Transcription termination is an essential step in transcription by RNA polymerase (RNAP) and crucial for gene regulation. For many bacterial genes, transcription termination is mediated by the adenosine triphosphate–dependent RNA translocase/helicase Rho, which causes RNA/DNA dissociation from the RNAP elongation complex (EC). Rho is an adenosine triphosphate (ATP)–dependent RNA translocase/helicase with 5′ → 3′ directionality. Rho forms a ring-shaped homo-hexameric complex, mediated by the CTD.

The type 1 and type 2 RNAP-Rho complexes both revealed the closed-ring Rho hexamer with RNA threaded in the central channel, but they have different Rho binding sites and orientations relative to RNAP. Our cryo-EM analysis also provided another Rho-RNAP complex (the type 2 complex), in which Rho binds near the DNA exit site of apo RNAP through its NTD side. In the type 2 complex, Rho is bound to RNAP in an inverted orientation, as compared with that in the type 1 complex. The Rho hexamer assumes a closed-ring conformation with RNA threaded through the Rho central channel and binds near the DNA exit site of RNAP through its NTD side. Four of the six Rho protomers are involved in the RNAP interaction: Rho protomers B and C contact the base part of the β-flap domain (residues β727 to β738), protomers C and D contact the jaw-lobe 1 domain, and protomer E contacts the clamp coiled-coil of RNAP. The T4L insertions into the NTD did not affect the RNA release activity of Rho. Moreover, the deletion of the RNAP β-flap tip, which is critical for the Rho-dependent RNA release, enhanced the formation of the type 2 complex. Therefore, the inverted Rho-binding mode in this complex is unlikely to be relevant to termination. The abundance of the type 2 complex in the cryo-EM particles suggests that Rho may preferentially bind apo RNAP in this alternative mode. Therefore, this complex could potentially resemble a posttermination state formed after the EC has released DNA and RNA.

>[6x]GPMRRKETLQETPLTYQELASKILPELHLLAQEAGIEGYKRMKKDQLIMALLERQTQGEGLRLVKGYLEISQDGYGFLTENLHNLESRVAIVSAGLIKQYALRAGDYVVGQARPPRENERYATLLKVEAVNNLDPEAAKNRPRFDELTPQFPDRQIRLETTPDELSTRVIDLLAPIGRGQRGLIVAPPKAGKTTLLKKIANAVLKNEPDIKVIVLLIDERPEEVTDFRESVQGAEVIASTFDEPPQNHIRVAEFVHERAKRIVEEGGHVMILLDSITRLARANNLVTPPTGRTLSGGLDSAALYFPKRFLGAARNIRGGGSLTILATALVETGSRMDDVIFEEFKGTGNMELHLSRRLEERRIFPAIDILKSGTRREELLLGEEVTHKMWLLRKVLADMDPAEAMEMLLARLARTKNNKEFLASLAAR;>[2x]MLDSKLKAPVFTVRTQGREYGEFVLEPLERGFGVTLGNPLRRILLSSIPGTAVTSVYIEDVLHEFSTIPGVKEDVVEIILNLKELVVRFLNPSLQTVTLLLKAEGPKEVKARDFLPVADVEIMNPDLHIATLEEGGRLNMEVRVDRGVGYVPAEKHGIKDRINAIPVDAVFSPVRRVAFQVEDTRLGQRTDLDKLTLRIWTDGSVTPLEALNQAVEILREHLTYFSNPQAAAVAAPEEAKEPEAPPEQEEELDLPLEELGLSTRVLHSLKEEGIESVRALLALNLKDLKNIPGIGERSLEEIKEALEKKGFTLKE;> MEIKRFGRIREVIPLPPLTEIQVESYRRALQADVPPEKRENVGIQAAFRETFPIEEEDKGKGGLVLDFLEYRLGEPPFPQDECREKDLTYQAPLYARLQLIHKDTGLIKEDEVFLGHIPLMTEDGSFIINGADRVIVSQIHRSPGVYFTPDPARPGRYIASIIPLPKRGPWIDLEVEPNGVVSMKVNKRKFPLVLLLRVLGYDQETLARELGAYGELVQGLMDESVFAMRPEEALIRLFTLLRPGDPPKRDKAVAYVYGLIADPRRYDLGEAGRYKAEEKLGIRLSGRTLARFEDGEFKDEVFLPTLRYLFALTAGVPGHEVDDIDHLGNRRIRTVGELMTDQFRVGLARLARGVRERMLMGSEDSLTPAKLVNSRPLEAAIREFFSRSQLSQFKDETNPLSSLRHKRRISALGPGGLTRERAGFDVRDVHRTHYGRICPVETPEGANIGLITSLAAYARVDELGFIRTPYRRVVGGVVTDEVVYMTATEEDRYTIAQANTPLEGNRIAAERVVARRKGEPVIVSPEEVEFMDVSPKQVFSVNTNLIPFLEHDDANRALMGSNMQTQAVPLIRAQAPVVMTGLEERVVRDSLAALYAEEDGEVAKVDGNRIVVRYEDGRLVEYPLRRFYRSNQGTALDQRPRVVVGQRVRKGDLLADGPASENGFLALGQNVLVAIMPFDGYNFEDAIVISEELLKRDFYTSIHIERYEIEARDTKLGPERITRDIPHLSEAALRDLDEEGVVRIGAEVKPGDILVGRTSFKGESEPTPEERLLRSIFGEKARDVKDTSLRVPPGEGGIVVRTVRLRRGDPGVELKPGVREVVRVYVAQKRKLQVGDKLANRHGNKGVVAKILPVEDMPHLPDGTPVDVILNPLGVPSRMNLGQILETHLGLAGYFLGQRYISPIFDGAKEPEIKELLAQAFEVYFGKRKGEGFGVDKREVEVLRRAEKLGLVTPGKTPEEQLKELFLQGKVVLYDGRTGEPIEGPIVVGQMFIMKLYHMVEDKMHARSTGPYSLITQQPLGGKAQFGGQRFGEMEVWALEAYGAAHTLQEMLTLKSDDIEGRNAAYEAIIKGEDVPEPSVPESFRVLVKELQALALDVQTLDEKDNPVDIFEGLASKR;> MKKEVRKVRIALASPEKIRSWSYGEVEKPETINYRTLKPERDGLFDERIFGPIKDYECACGKYKRQRFEGKVCERCGVEVTKSIVRRYRMGHIELATPAAHIWFVKDVPSKIGTLLDLSATELEQVLYFSKYIVLDPKGAILNGVPVEKRQLLTDEEYRELRYGKQETYPLPPGVDALVKDGEEVVKGQELAPGVVSRLDGVALYRFPRRVRVEYVKKERAGLRLPLAAWVEKEAYKPGEILAELPEPYLFRAEEEGVVELKELEEGAFLVLRREDEPVATYFLPVGMTPLVVHGEIVEKGQPLAEAKGLLRMPRQVRAAQVEAEEEGETVYLTLFLEWTEPKDYRVQPHMNVVVPEGARVEAGDKIVAAIDPEEEVIAEAEGVVHLHEPASILVVKARVYPFEDDVEVSTGDRVAPGDVLADGGKVKSDVYGRVEVDLVRNVVRVVESYDIDARMGAEAIQQLLKELDLEALEKELLEEMKHPSRARRAKARKRLEVVRAFLDSGNRPEWMILEAVPVLPPDLRPMVQVDGGRFATSDLNDLYRRLINRNNRLKKLLAQGAPEIIIRNEKRMLQEAVDALLDNGRRGAPVTNPGSDRPLRSLTDILSGKQGRFRQNLLGKRVDYSGRSVIVVGPQLKLHQCGLPKRMALELFKPFLLKKMEEKGIAPNVKAARRMLERQRDIKDEVWDALEEVIHGKVVLLNRAPTLHRLGIQAFQPVLVEGQSIQLHPLVCEAFNADFDGDQMAVHVPLSSFAQAEARIQMLSAHNLLSPASGEPLAKPSRDIILGLYYITQVRKEKKGAGLEFATPEEALAAHERGEVALNAPIKVAGRETSVGRLKYVFANPDEALLAVAHGIVDLQDVVTVRYMGKRLETSPGRILFARIVAEAVEDEKVAWELIQLDVPQEKNSLKDLVYQAFLRLGMEKTARLLDALKYYGFTFSTTSGITIGIDDAVIPEEKKQYLEEADRKLLQIEQAYEMGFLTDRERYDQILQLWTETTEKVTQAVFKNFEENYPFNPLYVMAQSGARGNPQQIRQLCGLRGLMQKPSGETFEVPVRSSFREGLTVLEYFISSHGARKGGADTALRTADSGYLTRKLVDVTHEIVVREADCGTTNYISVPLFQPDEVTRSLRLRKRADIEAGLYGRVLAREVEVLGVRLEEGRYLSMDDVHLLIKAAEAGEIQEVPVRSPLTCQTRYGVCQKCYGYDLSMARPVSIGEAVGIVAAQSIGEPGTQLTMRTFHTGGVAGAADITQGLPRVIELFEARRPKAKAVISEIDGVVRIEETEEKLSVFVESEGFSKEYKLPKEARLLVKDGDYVEAGQPLTRGAIDPHQLLEAKGPEAVERYLVEEIQKVYRAQGVKLHDKHIEIVVRQMMKYVEVTDPGDSRLLEGQVLEKWDVEALNERLIAEGKTPVAWKPLLMGVTKSALSTKSWLSAASFQNTTHVLTEAAIAGKKDELIGLKENVILGRLIPAGTGSDFVRFTQVVDQKTLKAIEEARKEAVEAKERPAARRGVKREQPGKQADYKDDDDK;> MAEPGIDKLFGMVDSKYRLTVVVAKRAQQLLRHGFKNTVLEPEERPKMQTLEGLFDDPNAVTWAMKELLTGRLVFGENLVPEDRLQKEMERLYPVEREE> TIFQFPQDFMWGTATAAYQIEGAYQEDGRGLSIWDTFAHTPGKVFNGDNGNVACDSYHRYE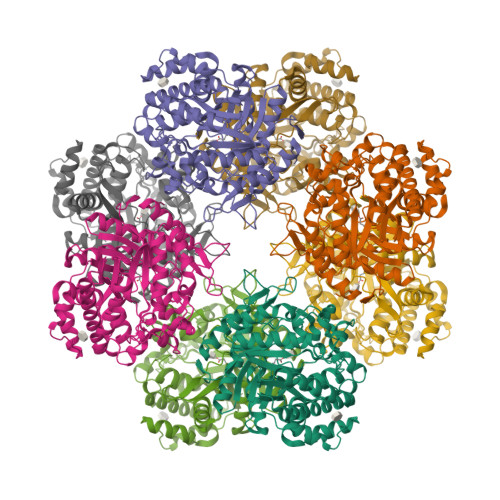EDIRLMKELGIRTYRFSVSWPRIFPNGDGEVNQEGLDYYHRVVDLLNDNGIEPFCTLYHWDLPQALQDAGGWGNRRTIQAFVQFAETMFREFHGKIQHWLTFNEPWCIAFLSNMLGVHAPGLTNLQTAIDVGHHLLVAHGLSVRRFRELGTSGQIGIAPNVSWAVPYSTSEEDKAACARTISLHSDWFLQPIYQGSYPQFLVDWFAEQGATVPIQDGDMDIIGEPIDMIGINYYSMSVNRFNPEAGFLQSEEINMGLPVTDIGWPVESRGLYEVLHYLQKYGNIDIYITENGACINDEVVNGKVQDDRRISYMQQHLVQVHRAIHDGLHVKGYMAWSLLDNFEWAEGYNMRFGMIHVDFRTQVRTPKQSYYWYRNVVGNNWLETRR>[2x]MAHHHHHHVGTMENENKPNVANFEAAVAAKDYEKACSELLLILSQLDSNFGGIQEIEFEYPAQLQDLEQEKIVYFCTRMATAITTLFSDPVLEISDLGVQRFLVYQRWLALIFASSPFVNADHILQTYNREPNRKNSLEIHLDSSKSSLIKFCILYLPESNVNLNLDVMWNISPELCASLCFALQSPRFIGTSTAFNKRATILQWFPRHLDQLKNLNNIPSAISHDVYMHCSYDTSVNKHDVKRALNHVIRRHIESEYGWKDRDVAHIGYRNNKPVMVVLLEHFHSAHSIYRTHSTSMIAAREHFYLIGLGSPSVDQAGQEVFDEFHLVAGDNMKQKLEFIRSVCESNGAAIFYMPSIGMDMTTIFASNTRLAPIQAIALGHPATTHSDFIEYVIVEDDYVGSEECFSETLLRLPKDALPYVPSALAPEKVDYLLRENPEVVNIGIASTTMKLNPYFLEALKAIRDRAKVKVHF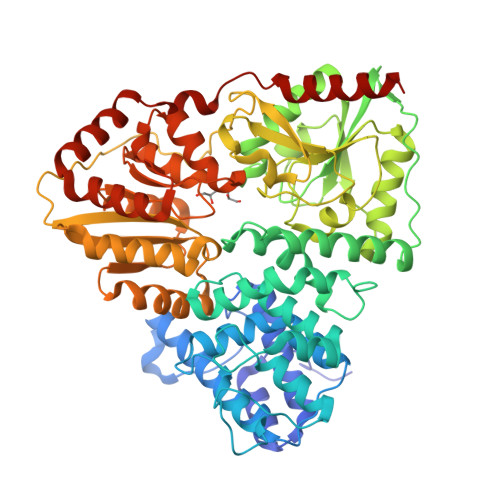HFALGQSNGITHPYVERFIKSYLGDSATAHPHSPYHQYLRILHNCDMMVNPFPFGNTNGIIDMVTLGLVGVCKTGAEVHEHIDEGLFKRLGLPEWLIANTVDEYVERAVRLAENHQERLELRRYIIENNGLNTLFTGDPRPMGQVFLEKLNAFLKEN>RSPWPSNMKQFCKISVWLQQHDPDLLEIINNLCMLGNLSAAKYKHGVTFIYPKQAKIRDEIKKHAY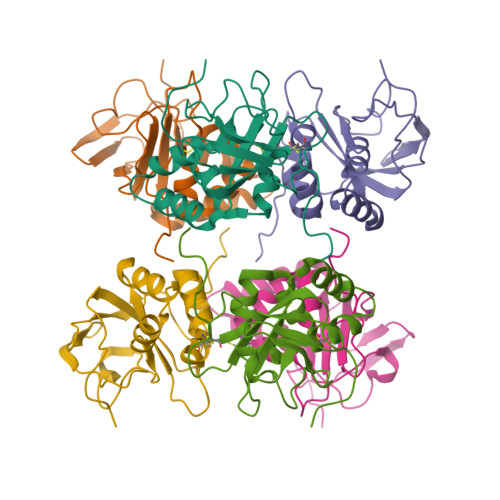SNDPSQAIKTLESLILPFYIPTPAEFTGEIGSYTGVKLEVEKTEANKVILKNGEAVLVPAADFKPFPDRRLAVWIMESGSMPLEGPPYKRKKEGGGNLESRGPFEGKPIPNPLLGLDSTRTGHHHHHH[2x]N-(R-CARBOXY-ETHYL)-ALPHA-(S)-(2-PHENYLETHYL) 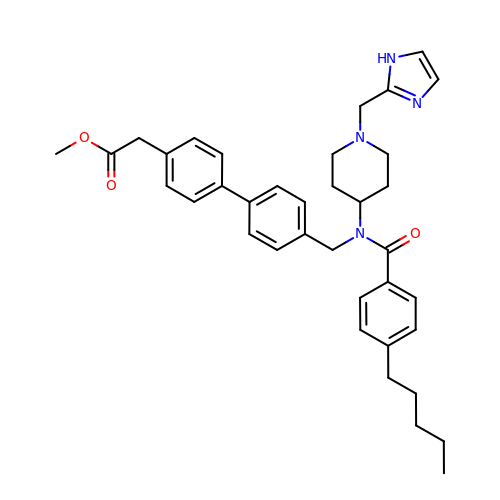| C37 H44 N4 O3 | JJVQUUYZGJWBPW-UHFFFAOYSA-N(2E)-1-[(6-chloropyridin-3-yl)methyl]-N-nitroimidazolidin-2-imine | C9 H10 Cl N5 O2 | 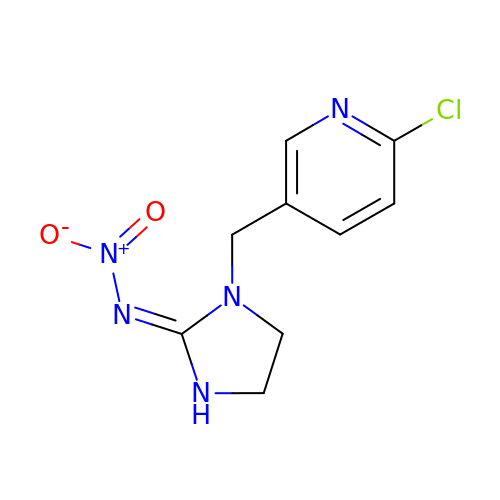YWTYJOPNNQFBPC-UHFFFAOYSA-N>MFGRKKGDVIDAGAELERAEQERIEGEYGASELASERRPHTPGARTLLMVLLCVIAVVLVTLSYKAYKVRGVVEDDDAQPQQVVRQVIPGYTPRPIRPEPENVPEPPQPTTSVPAIQPAPVTQPVRPQPTGPREKTPYELARERMLRSGLTAGSGGGEDLPRPQGGDVPAGGLMGGGGGGGELAEKLQPMRLSGSSAGRLGNRDMLITQGTQLDCVLETRLVTTQPGMTTCHLTRDVYSTSGRVVLLDRGSKVVGFYQGGLRQGQARIFVQWSRIETPSGVVINLDSPGTGPLGEAGLGGWIDRHFWERFGGAIMISLIGDLGDWASRQGSRQGDNSIQFSNTANGVESAAAEALRNSINIPPTLYKNQGERVNILVARDLDFSDVYSLESIPTK[16x];>MKKLAIVALLASLHAVPALALDVPSSSRYDHRIRYVTYNPADVVQVDTVLGVATHIMLEEGEQYLTHAFGDSEAYAFARKGRHIFIKPQAELANTNLIVVTDRRSYKFRLQMRNDRNGAMYELAFRYPDTQARQTREANARAAVEAAFEQRVGAYYNLKYMMSGDKDIAPVNAWDDGRFTYFKFSANADLPSIYFVDAEGNESLVPRTTVGSSNNIIAVHKVNPKWMIRLGNRALAIFNEAYDPNGVPNDTGTASPAVRRVNKGGN[16x];>[14x]MKTIIFAILMTGLLSACASAPKPKQPSDFNREPVNKTVPVEIQRGAL

Conjugative type IV secretion systems (T4SS) mediate bacterial conjugation, a process that enables the unidirectional exchange of genetic materials between a donor and a recipient bacterial cell. Bacterial conjugation is the primary means by which antibiotic resistance genes spread among bacterial populations. The recent cryo-electron microscopy (cryo-EM) structure of the conjugative Type 4 Secretion System (T4SS) encoded by the plasmid R388 revealed that the remaining VirB proteins form a large assembly organised into four sub-complexes: the outer membrane core complex (OMCC), the stalk, the arches and the inner membrane complex (IMC). Previously, we solved the cryo-electron microscopy (cryo-EM) structure of a conjugative T4SS. In this article, based on additional data, we present a more complete T4SS cryo-EM structure than that published earlier.

Further analysis employing 3D classification (Fig. EV1) reveals a degree of heterogeneity in the positioning of the two extra TrwF/VirB9NTD-TrwE/VirB10NTD sub-complexes within the I-layer. We obtained three distinct OMCC structures, each characterised by a unique arrangement of the two extra sub-complexes in the I-layer. Aligning the structures of these three I-layer conformations using the O-layer as the reference underscores how the variability in the positions of the two extra I-layer complexes impacts the overall I-layer structure. Although the structure of each complex forming the I-layer do not change significantly (RMSD of 1.06 Å), a shift between corresponding complexes in the superposition of conformations A and B or A and C is observed. In both, this shift changes in magnitude, being maximal in the superposition involving the second extra sub-complex (that in orange in Fig. 2C i.e. complex 10 in the A versus B superposition and complex 11 in the A versus C superposition) and, intriguingly, being minimal in the complexes opposite (complex 2 in the A versus B superposition and complex 3 in the A versus C superposition). Thus, the insertion of extra complexes occurs at various positions in the I-layer, resulting in structural adjustments that propagate over the entire I-layer.Here, we report the structural and biochemical studies of the highly conserved C962R protein of ASFV, showing that C962R is a multidomain protein. The N-terminal AEP domain is responsible for the DNA polymerization activity, whereas the DNA unwinding activity is catalyzed by the central SF3 helicase domain. The middle PriCT2 and D5_N domains and the C-terminal Tail domain all contribute to the DNA unwinding activity of C962R. C962R preferentially works on forked DNA, and likely functions in Base-excision repair (BER) or other repair pathway in ASFV.

To gain more insights into the assembly of C962R, the apo protein was subjected to 300 kV cryo-EM analysis. Three-dimensional (3D) reconstruction and refinement further confirmed that C962R assembles into dodecamer, which is consistent with the size-exclusion chromatographic profile, AUC and SEC-MALS analysis. C962R dodecamer is formed by two ring-shaped hexamers. The diameter of the outer ring is about 140 Å; and, the height of the C962R dodecamer is approximately 290 Å. The C962R structure was refined up to an overall resolution of 3.67 Å. Although it cannot be predicted by the sequence, the structure revealed a compact domain for the C-terminal Asp833-His910 region. The domain is of α/β fold in nature and was termed Tail domain hereafter. Dodecamerization of C962R is mediated by the AEP domains, mainly through the hydrophobic interactions between the side chains of His120 and Tyr238 residues. In the apo structure, the six Tail domains are symmetrically arranged along the central axis; the diameter of the inner ring is approximately 50 Å. In the absence of DNA, C962R exists as a dodecamer with the AEP domains located at the interface of the two hexamers.

>[12x]GSMREESWEEHDTIQLTAQRKYLAEVQALETLLARELSVFLTEPGSKKTNIINRITGKTYALPSTELLRFYEHLEQCRKQGALMYFLERQGTYSGLMLDYDLKLNTNAAPSLESSVLSRLCHRIFVHIKNSSVLPEGSHKIHFFFTLKPEAVQGKYGFHVLIPGLKMAASTKKSIIASLQHDATVQKILHEQGVANPESCLDPHSASVPSLLYGSSKLNHRPYQLKTGFELVFDSSDPDYIPIHQIKNIESYNLVSELSLTNEQGSLVRPVYCAADIAAEKEEEIPADDHSLSILMLHDPEARYLHKILNLLPPEYYVEYPLWSNVVFALANTSANYRPLAEWFSQKCPEKWNTGGKEKLEKLWNDASRHTEKKITKRSIMYWAHKHAPQQYKEIVEQGYFSILAEYVYSYNGTLEHYMIAKVIYAMMGNKFVVDVDSNGKYVWFEFVLPGQPMNQGEIWKWRKEVNPDELHIYISENFSRVMDRITEHIKYHLSQPHETNILNYYKKLLKAFERSKSKIFNDSFKKGVIRQAEFLFRQRSFIQTLDTNPYLLGVGNGVLSIETIPAKLINHFHEHPIHQYTHICYEPFNPENPWTKLLLNALQDIIPELDARLWIMFYLSTAIFRGLKEALMLLWLGGGCNGKTFLMRLVAMVLGDHYASKLNISLLTSYRETAEKPNSAFMRLKGRGYGYFEETNKSEILNTSRLKEMVNPGDVTARELNQKQESFQMTATMVAASNYNFIIDTTDHGTWRRLRHYRSKVKFCHNPDPNNSYEKKEDPRFIHEYIMDPNCQNAFFSILVYFWEKLQKEYNGQIKKVFCPTIESETEAYRKSQDTLHRFITERVVESPSAETVYNLSEVVTAYAEWYNANINVKRHIALELSQELENSVLEKYLQWSPNKTRILKGCRILHKFETLQPGESYIGVSSTGTLLNTPICEPKNKWWEWSPNPSAPPEKEASAPTP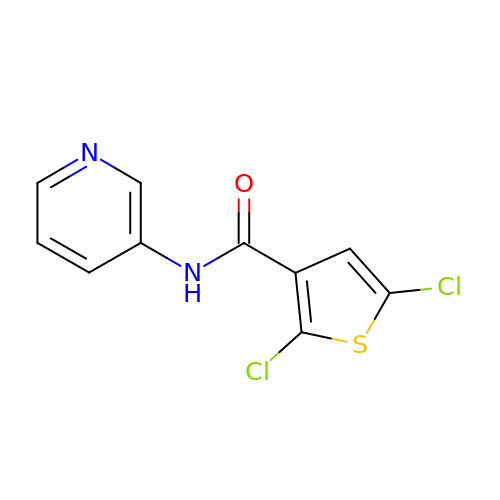2,5-dichloro-N-(pyridin-3-yl)thiophene-3-carboxamide | C10 H6 Cl2 N2 O S | XUXVQIKOGRNZPD-UHFFFAOYSA-N> GSHMAKTYDYLFKLLLIGDSGVGKTCVLFRFSEDAFNSTFISTIGIDFKIRTIELDGKRIKLQIWDTAGLERFRTITTAYYRGAMGIMLVYDITNEKSFDNIRNWIRNIEEHASADVEKMILGNKCDVNDKRQVSKERGEKLA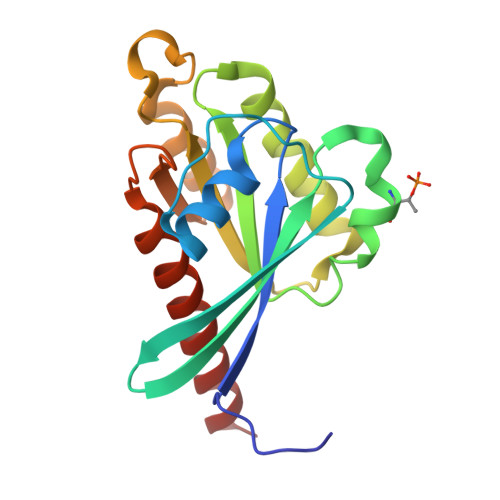LDYGIKFMETSAKANINVENAFFTLARDIKAKMDKKLEGNS> GPLGSMSSIGLAHNVTILGSGETTVVLGHGYGTDQSVWKLLVPYLVDDYKVLLYDHMGAGTTNPDYFDFDRYSSLEGYSYDLIAILEEFQVSKCIYVGHCMSSMAAAVASIFRPDLFHKLVMISPTPRLINTEEYYGGFEQKVMDETLRSLDENFKSLSLGTAPLLLACDLESAAMQEYCRTLFNMRPDIACCITRMICGLDL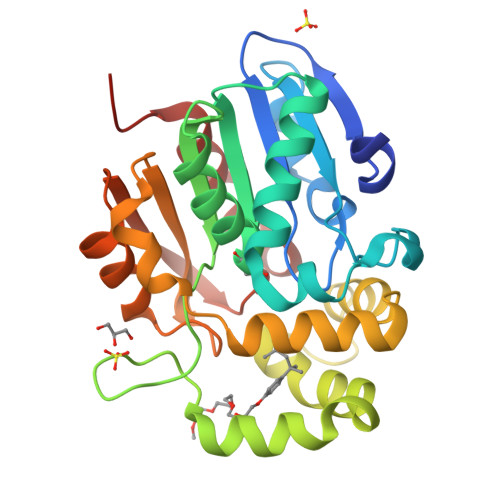RPYLGHVTVPCHIIQSSNDIMVPVAVGEYLRKNLGGPSVVEVMPTEGHLPHLSMPEVTIPVVLRHIRQDITDH A common step during their assembly is polyketide trimming, which Afyg1p, Wdyg1p, and PlAntI catalyze. In summary, the N‐ and C‐domains in all three enzymes are oriented in a back‐to‐back fashion forming an interface that encloses the intramolecular binding cavity next to the active site. The catalytic triad is formed exclusively by the α/β‐hydrolase domain with the nucleophilic serine located in the consensus GXSXG esterase motif. The resulting Ser‐His‐Asp network is perfectly aligned with distances in the range of 2.5–2.8 Å between the active‐site residues.

In contrast, in the zoonotic pathogen Wangiella (Exophiala) dermatitidis (Wd), the acetyl group of the hexaketide 2‐acetyl‐1,3,6,8‐tetrahydroxynaphthalene (ATHN), WdPKS product, is hydrolyzed by the Afyg1p homolog Wdyg1p. Single‐wavelength anomalous diffraction (SAD) was performed to obtain experimental phases for Afyg1p, which was used as a model for Patterson search calculations of the Wdyg1p structure. The N‐domains exhibit an α‐helix bundle, whereas the C‐domains adopt a classical α/β‐hydrolase topology. The amino acid sequences of Afyg1p and Wdyg1p have 40% sequence identity, which explains the similarity in their overall folds and active‐site residues (rmsd = 1.1 Å over 382 Cα‐atoms, Figure 3b). Although both enzymes differ significantly from PlAntI in terms of catalysis and primary sequence, their superposition shows a perfect match of secondary structure elements (rmsd = 1.6 Å over 244 Cα‐atoms for Afyg1p and rmsd = 1.8 Å over 247 Cα‐atoms for Wdyg1p). Interestingly, both hydrolases provide a hydrophobic tunnel beside the naphthalene specificity pocket. The 400 Å3 cavity of Wdyg1p is confined by the amino acids Thr257, Leu304, Leu308, and Phe353, which could accommodate an acetyl group. Hydrolysis of the Ser256‐bound acetoacetyl group finally restores the catalytic center and releases the products THN and 3‐oxobutanoate. This mechanism is most likely transferable to Wdyg1p due to the high similarity of their active‐site architectures and the GLDG binding motifs. Notably, the entire reaction in the hydrolases Afyg1p and Wdyg1p happens in an open state.

>[2x]MGWSHPQFEKENLYFQGSATEKYYIRDAITKPAVHHESYQKLWETKWKKPCEMGVYPFMFGSIKDFEPVAQEIIKKGLKEPYDWDEYAQMYFPKAEELAKIAEEAEAAGEKEKASEYYLRSSAVYRISRFPTPRSEKQKYAWRKGCEVFYKGAALMEYPIKEVRIPHKHGIEGEGDVVPVNFLLPPNASETSPVPCVLIITGLDGYRTELAVWQQGWRSKGVATVIAEIPGTGDSPALRQDPTSPDRQWSSVLDWIESQKAVDSKKIVAWGFSTGGYYALRMAHTHKDRLLATISLGGGAHHMFDREWLEHANKLEYPFDLSNTLAYKFGYPDLESFIEESSKFSLLNDGTLQKPCTKVLLVNGNDDEIFPIDDMFVSLENGQPKLARMVKGKKHMGEPESFSIILEWIHKLLGLDGKIKEQLAMIPSRTK> XAALAQIKKE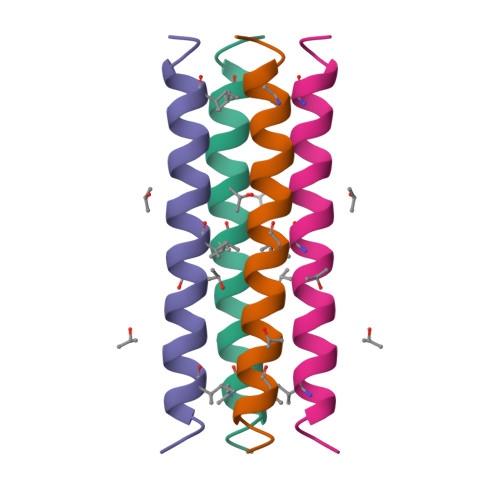IAYLLAKIKAEILAALKKIKQEIAX3-{[2-({N-[(2S)-2-hydroxy-3,3-dimethyl-4-(phosphonooxy)butanoyl]-beta-alanyl}amino)ethyl]sulfanyl}-3-oxopropanoic acid | C14 H25 N2 O10 P S | 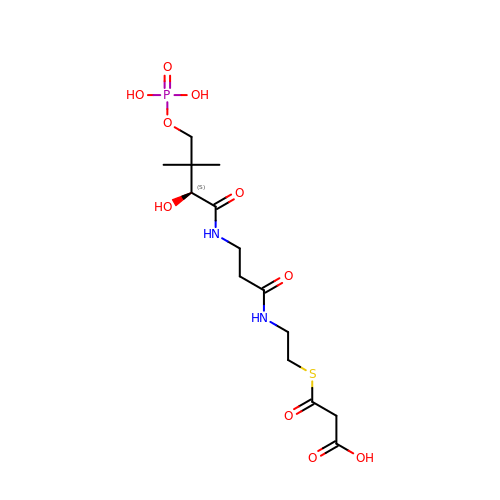RNFWAFOKCVKQGB-GFCCVEGCSA-N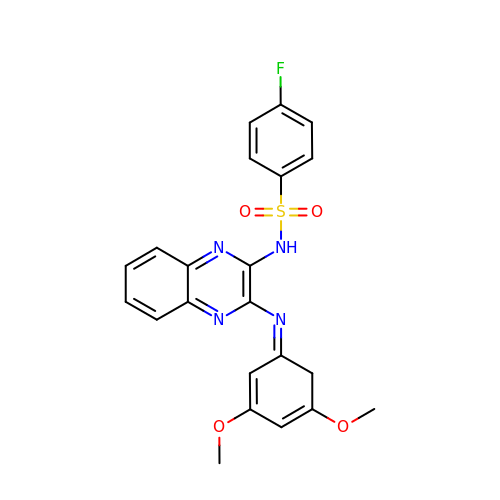N-(3-{[(1Z)-3,5-DIMETHOXYCYCLOHEXA-2,4-DIEN-1-YLIDENE]AMINO}QUINOXALIN-2-YL)-4-FLUOROBENZENESULFONAMIDE | C22 H19 F N4 O4 S | WCHXKEIXBGDHMP-BUVRLJJBSA-N>LSLFYGVS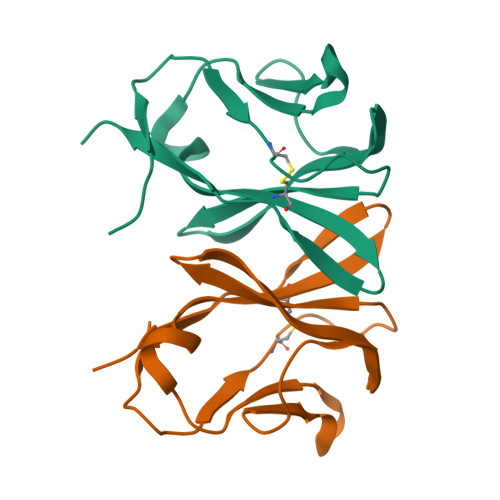ARIYKEGEKVQVDCDLKQSGTLTFWFRINSKGADYLFSVKSADIKENDLNSEHYTVNTNSGKVQLDIKSFKKKTDSGVYVCAAMNSNKLFFGGLTRIEGEPDPTTIPPKIATTKPLPVTA[2x]(2R,3R,4S,5S)-2-(6-amino-9H-purin-9-yl)-5-{[(3-nitrobenzyl)disulfanyl]methyl}tetrahydrofuran-3,4-diol 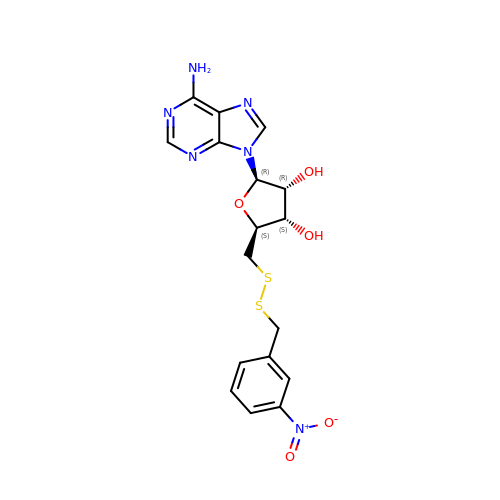| C17 H18 N6 O5 S2 | UWYQTICCMFSWOE-LSCFUAHRSA-N>MSNATKFGKVAVLLGGKSAERAVSLDSGQAVLDALLRSGVQAEAFDPQDRSVTELVNYDRAFIVLHGRGGEDGQIQGVLEWLNIPYTGTGVQGSAIGMDKVKTKQIWQGSDLPTAPYRIITKETDLDSVIAELGLP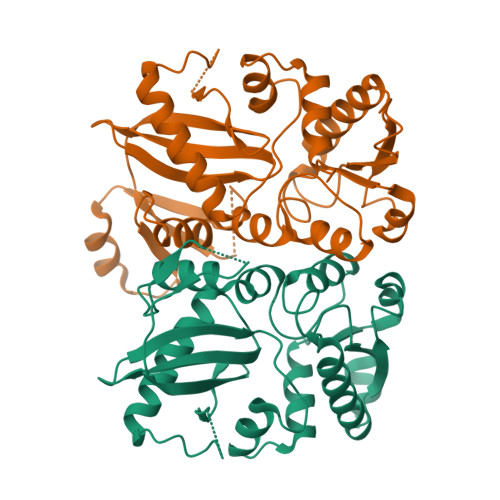VIIKPVHEGSSVGMSKVEKAEDFAAAIEKATQHDAVVMAEKWITGREFTISFLNGQPLPVIRLQPPADVAFYDYEAKYQRNDVEYGIPCGLSETEEKKLQALCLRAFQAVGAEGWGRIDAMQDEQGNFWLLEVNTVPGMTSHSLVPKAAKAVGYSFDELCVAILEQTLEGTA[6x]> MTAPEQTFRNKKQRKQQVKLRKPGFAVAKYVRMSPRKVRLVVDVIRGKSVQDAEDLLRFIPRSASEPVAKVLNSAKANALHNDEMLEDRLFVKEAYVDAGPTLKRLIPRARGSANIIKKRTSHITIIVAEKGNK;> MAKHPVPKKKTSKSKRDMRRSHHALTAPNLTECPQCHGKKLSHHI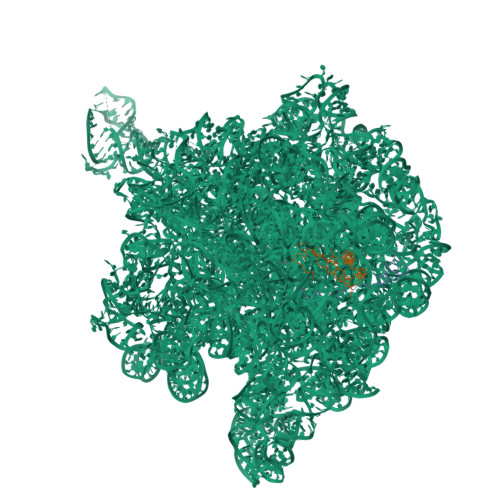CPNCGYYDGRQVLAV> MEEGARHRNNTEKKHPGGGESDASPEAGSGGGGVALKKEIGLVSACGIIVGNIIGSGIFVSPKGVLENAGSVGLALIVWIVTGFITVVGALCYAELGVTIPKSGGDYSYVKDIFGGLAGFLRLWIAVLVIYPTNQAVIALTFSNYVLQPLFPTCFP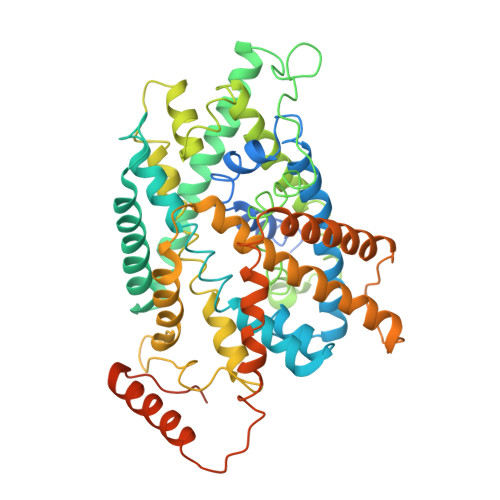PESGLRLLAAICLLLLTWVNCSSVRWATRVQDIFTAGKLLALALIIIMGIVQICKGEYFWLEPKNAFENFQEPDIGLVALAFLQGSFAYGGWNFLNYVTEELVDPYKNLPRAIFISIPLVTFVYVFANVAYVTAMSPQELLASNAVAVTFGEKLLGVMAWIMPISVALSTFGGVNGSLFTSSRLFFAGAREGHLPSVLAMIHVKRCTPIPALLFTCISTLLMLVTSDMYTLINYVGFINYLFYGVTVAGQIVLRWKKPDIPRPIKINLLFPIIYLLFWAFLLVFSLWSEPVVCGIGLAIMLTGVPVYFLGVYWQHKPKCFSDFIELLTLVSQKMCVVVYPEVERGSGTEEANEDMEEQQQPMYQPTPTKDKDVAGQPQP>[2x]MGHHHHHHMNSVKNEENTSKEHAPDKIVLDHAFGQTILDKKPERVATIAWGNHDVALALGIVPVGFSKANYGVSADKGVLPWTEEKIKELNGKANLFDDLDGLNFEAISNSKPDVILAGYSGITKEDYDTLSKIAPVAAYKSKPWQTLWRDMIKIDSKALGMEKEGDELIKNTEARISKELEKHPEIKGKIKGKKVL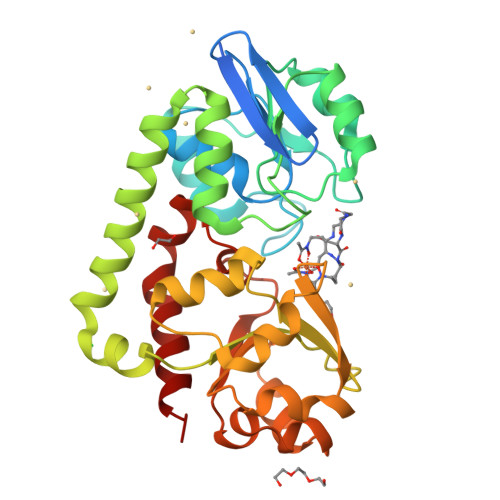FTMINAADTSKFWIYTSKDPRANYLTDLGLVFPESLKEFESEDSFAKEISAEEANKINDADVIITYGDDKTLEALQKDPLLGKINAIKNGAVAVIPDNTPLAASCTPTPLSINYTIEEYLNLLGNACKNAK>PAAELEARQFDPDSFKNKWLELHNNERTTRQLDSLEWDGDLAWKAQQVATQCNVDNPQLWGDNGASFNIGRYTKEQAFAEWTATSGSFPDDRSIPWQRIVANSAQKVGCGEATCVLEGDMAYTVNVCYYDPPLSDYYTNAGDNVRVPSLALLNLDLTTPFCNLPVNGSNDLDIRE[7x]

We present in this report the structure of MpPR-1i, a SCP/TAPS protein expressed by M. perniciosa during biotrophic stage of WBD, in basidiomes, and in monokaryotic mycelia. MpPR-1 proteins are homologues of plant pathogenesis–related-1 (PR-1) proteins that were first identified over a century ago as important for defense against fungi and parasites. PR-1 proteins are members of the eukaryotic CAP (cysteine-rich secretory protein/antigen 5/pathogenesis related-1) or SCP/TAPS (Sperm-coating protein/Tpx/antigen 5/pathogenesis related-1/Sc7) superfamily of proteins, which has been implicated in biological processes like reproduction, fungal virulence, cellular defense, and immune evasion. Each monomer of MpPR-1i has a conserved alpha-beta-alpha sandwich topology made up of 3 β strands sandwiched between two helical domains, connected by loops.

The structure was refined and extended to higher resolution, using a 2.43 Å native data set. There are seven monomers in the asymmetric unit, which form a pseudo seven fold screw axis when viewed along the diagonal of the cell. The MpPR-1i crystal has very high solvent content, ~70%, which is clearly demonstrated by the solvent channel in the crystal packing viewed along a cell dimension. The main chains of the MpPR-1i monomers are very similar with rmsd ranging between 0.19 Å to 0.27 Å. The most variable regions between the monomers are loop regions, notably the solvent exposed loop connecting the two longest β-stands, as well as the N- and C-termini loops. MpPR-1i forms a unique crystallographic heptamer, which likely does not have any functional relevance as MpPR-1i forms monomers in solution. MpPR-1i, like SmVAL4, lacks the tetrad that binds divalent cations in other SCP/TAPS proteins. This explains why MpPR-1i does not bind Zn2+ used in the crystallization solution. Structural comparisons with tablysin-15, a palmitate binding CAP protein, showed that MpPR-1i has a similar cavity sufficiently large and open to accommodate palmitate or similar lipids. The shortened length of the CBM loop significantly reduces the size of the sterol binding cavity, rendering it barely large enough to accommodate dioxane and definitely too small to accommodate cholesterol.> MRKSLVALLLLAASGLAQAQVDLREGHPDRYTVVRGDTLWDISGKFLRQPWKWPELWHANPQIQNPHLIYPGDTLSLVYVDGQPRLVLNRGESRGTIKLSPKIRSTPIAEAIPTIPLDKINSFLLANRIVDDEKTFTSAPYIVAGNAERIVSGTGDRIYARGKFADGQPAYGIFRQGKVYIDPKTKEVLGINADDIGGGEVVATEGDVATLALTRTTQEVRLGDRLFPTEERAVNSTFMPGEPSREVKGEIIDVPRGVTQIGQFDVVTLNRGQRDGLAEGNVLAIYKVGETVRDRVTGESVKIPDERAGLLMVFRTYKKLSYALVLMASRP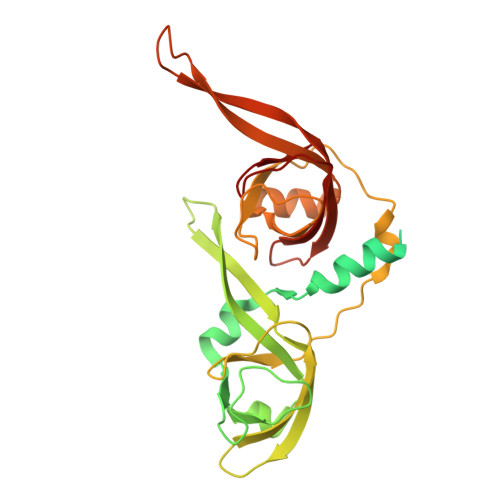LSVTDRVQNP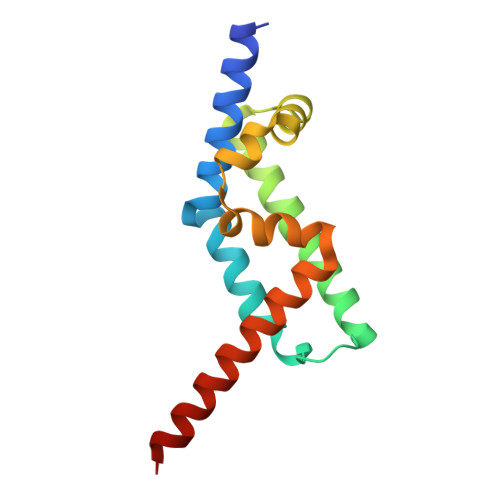> GPMAAEEEDEVEWVVESIAGFLRGPDWSIPILDFVEQKCEVFDDEEESKLTYTEIHQEYKELVEKLLESYLKEIGINEDQFQEACTSPLAKTRTSQAILQPVLAAEDFTIFKAMMVQKNIEMQLQAIRIIQERNG> QWNSRYSYNQLKNKDSLIMFLVEIFRSLFVSNCIDKNIDNVLLSIEEMFIDHYYNPQHSRLKYLIDDVGIFFTKLPITKAFHTYNKKYRITKRLYAPPTFNEVRHILNLAQILSLEEGLDLLTFDANETLYPDGHDFNDEVLASYISCLLKKMNIAIVTAASYNNDAEKYQKRLENLLKYFSKHNIKDGSYKNFYVMGGESNYLFKCNEEAT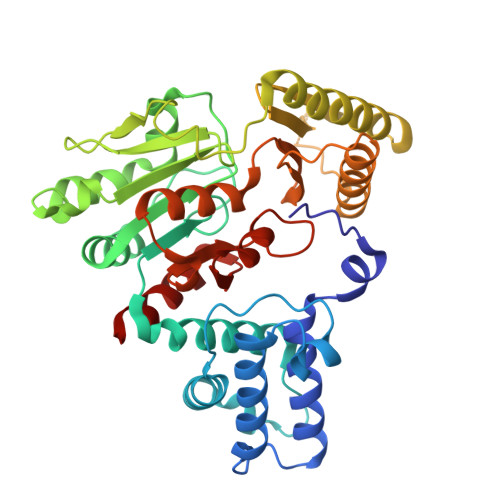LYSVPENEWRHYKKFVDYDTVQEILNISEKCLEKVIKDFGLCAQIQRKEKSIGLVPNKIPSLNIKNEQKNYMIKYEVLEEAVIRIKKEIIKNKITAPYCAFNGGQDLWVDVGNKAEGLLILQKLLKIQKKKCCHIGDQFLHSGNDFPTRFCSLTLWVSNPQETKACLKSIMHL>MNTIAWLGRLVIERIRGIGVAALMLLQIIFSLPSAGGFGRFVYQMHRVGVMSLLIITVSGLFIGLVLGLQGYSILVNVGSESMLGTMVSLTLLRELAPVVAALLFAGRAGSALTAEIGSMKQSEQLASMEMIGVDPLKQIVSPRLWAGIVSLPMLTVIFAAIGIVGGKLVGVDFLGVDEGSFWSGMQNNVQFGHDVVNGIIKSIVFALLCTWIAVFQGYACDPTPEGIATAMTRTVVYSSLCVLGFDFVLTAVMFGGI[2x];>[2x]MMNNKTPLSTQSLIEVKNLSFNRGERVIYDNISLNIRRGQITAIMGPSGTGKTTLLRLIGGQLVPDQGEVLLDGKDIAQMSRQELFAARARMGMLFQSGALFTDMSVYENVAFPIRAHTKLSENLIAELVALKLESVGLRGTEQLMPTELSGGMNRRVALARAIALDPDLIMYDEPFAGQDPIVKGVLTRLIRSLREALDLTTIIVSHDVPETLSIADYIYVVAEGKIQGEGTPEELQAYASPFVKQFLTGSAEGPVEYQFSHQAYLDNEVRP;>VVQYLNQELVVSGKIDFENAEQQYQAGLAIIKKQTSFPLIVDLKQLEHGNTLALAVLVQWLRQTPQKSGLHFKNVPEKMLKIIQACHLQEDLHLVLEHHHHHH[2x];>MKSRTSELAVGIFVIIFGIALFFLAMKVSGLVGTNLSDGYTMKAQFDNVNGLKPRAKVTMSGVTIGRVDSITLDPVTRLATVTFDLDGKLTSFNAEQLKEVQKNALDELRYSSDYTQATPAQQKTMEQQLISNMNSITSIDEDAYIMVATNGLLGEKYLKIVPGGGLNYLKRGDTISNTQGTMDLEDLISKFITGGGAGKVAAGSSSAEEKAPASTDSSAQPSFVE[6x]

The MlaFEDB complex is an ATP-binding cassette transporter to actively translocate the phospholipids between the inner membrane and the periplasmic protein MlaC4,5. The MlaFEDB-mediated glycerophospholipid (PL) transport was reported to play an important role in maintaining the integrity of the lipid membrane. Consistent with the previous reported low-resolution A. baumannii MlaFEDB map8 and our E. coli MlaFEDB map9 (EMD-30355), the MlaF (cytoplasmic nucleotide-binding domain, NBD), MlaE (transmembrane domain), MlaD (periplasmic phospholipid-binding domain), and MlaB (cytoplasmic auxiliary domain) subunits are assembled in a stoichiometry of 2:2:6:2. In summary, we characterize four structures of the A. baumannii MlaFEDB complex in nucleotide-free and vanadate-trapped conformations using single-particle cryo-EM.

To understand the mechanism of glycerophospholipid translocation coupled with the conformational change, distinct conformations of MlaFEDB were trapped using sodium ortho-vanadate. Vanadate acts as a potent inhibitor of ATPase by forming an ADP–vanadate complex that mimics the intermediate state formed during hydrolysis. Three individual conformations were classified and refined to 4.0, 3.6, and 4.0 Å, and were named Vtrans1, Vtrans2, and Vclose, respectively. All three structures display bound nucleotides at the ATP-binding sites. However, the maps are of insufficient quality to distinguish between ADP, ATP, and ADP–vanadate. Comparison of Vtrans1 and Vtrans2 to nucleotide-free structure shows the conformational rearrangement of the MlaD. MlaD hexametric ring rotates clockwise at different levels, whereas MlaFEB remains unchanged. The three vanadate-trapped structures of MlaFEDB reveal different levels of conformational rearrangement of MlaD and MlaE coupled with nucleotide binding and glycerophospholipid translocation.>MSVVLPVAKRGEDILKLIAAPVSANELNSNWLYQLAD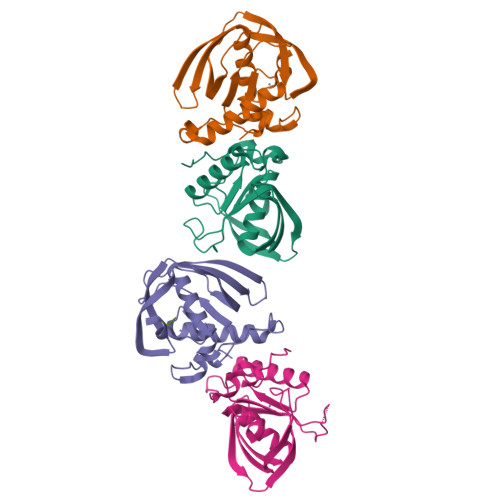AMHATMLERNGVGIAAPQVYISKRVIIVASRPNPRYPDAPEMNAVVMVNPEILEFSSEMCLGEEGCLSVPDERGQVERAEMVKVKYLTLQGEMVETVFQGFPARIVQHEVDHLNGILFVERIS[4x];> MAS>GPAVPRMVVLHSLLGMAVLIAIAVLLSTDRKAINIRTVAGAFLIQVALGALVLYVPQGRDMLGEASKTISNVIAYGNNGVDFLFGGLVSEKMFEVFGGGGFVFALRVLPMIVFFSSLMAVLYYIGVMQLLIKVIGGFLQKMLGTSKAESMSAAANIFVGQTEAPLVVRPYIRRMTESELFAVMSGGLASVAGSVLAGYVQMGVPLPYLIAASFMAAPGGLLFAKLLVPETERTQNDAEVLAENEDEKPTNVIDAAASG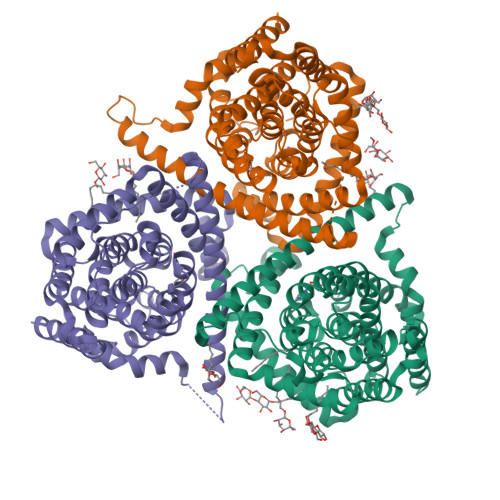AVTGAQIAIAVGASLLAFVALIAMINGIIGGVGGWFGHGDLTLQAILGWLFSPLAWVIGVPWSEAGIAGSLIGQKVVINEFVAYSEFVKYLKPEAAVQLSDTTKAIISFALCGFANLGSIAVLVGGLSIMAPKRRKDVARLGIKAVVAGSLSNLMSAVIAGLFTGLSGASVLG[3x]>DCHLSDMLQQLHSVNASKPSERGLVRQEEAEDPACIPIFWVSKWVDYSDKYGLGYQLCDNSVGVLFNDSTRLILYNDGDSLQYIERDGTESYLTVSSHPNSLMKKITLLKYFRNYMSEHLLKAGANITPREGDELARLPYLRTWFRTRSAIILHLSNGSVQINFFQDHTKLILCPLMAAVTYIDEKRDFRTYRLSLLEEYGCCKELASRLRYARTMVDKLLSS[3x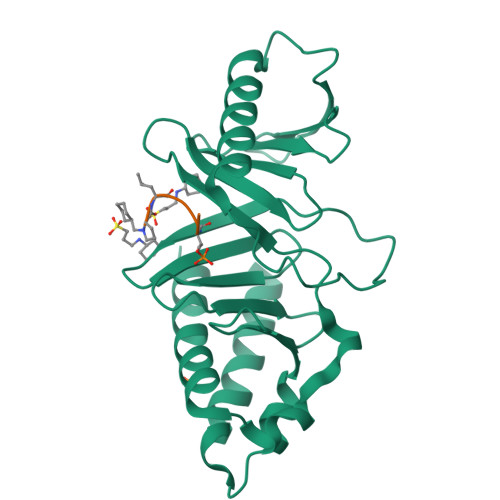]> MIEKSQACHDSLLDSVGQTPMVQLHQLFPKHEVFAKLE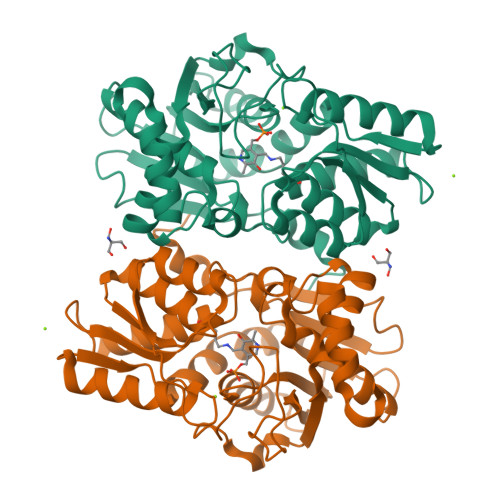YMNPGGSMKDRPAKYIIEHGIKHGLITENTHLIESTSGNLGIALAMIAKIKGLKLTCVVDPKISPTNLKIIKSYGANVEMVEEPDAHGGYLMTRIAKVQELLATIDDAYWINQFANELNWQSHYHGAGTEIVETIKQPIDYFVAPVSTTGSIMGMSRKIKEVHPNAQIVAVDAKGSVIFGDKPINRELPGIGASRVPEILNRSEINQVIHVDDYQSALGCRKLIDYEGIFAGGSTGSIIAAIEQLITSIEEGATIVTILPDRGDRYLDLVYSDTWLEKMKSRQGVKSE>TPDCVTGKVEYTKYNDDDTFTVKVGDKELFTNRANLQSLLLSAQITGMTVTIKTNACHNGGGFSEVIFR[5x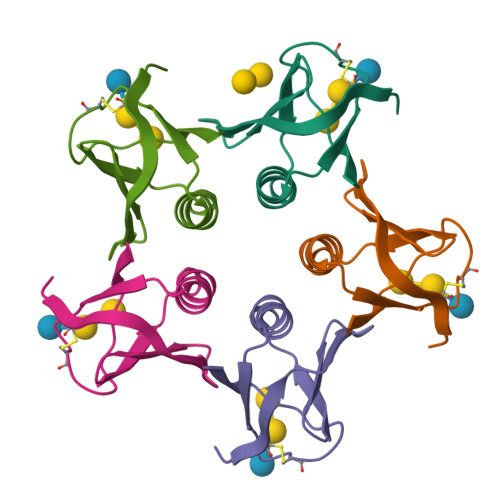]(1-{[(4R,6S)-8-chloro-6-(2,3-dimethoxyphenyl)-4H,6H-pyrrolo[1,2-a][4,1]benzoxazepin-4-yl]acetyl}piperidin-4-yl)acetic 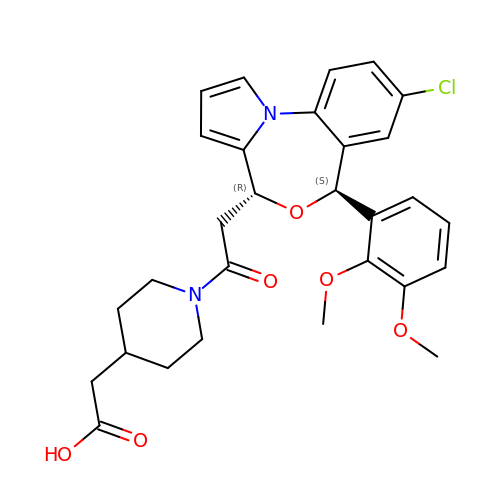acid | C29 H31 Cl N2 O6 | MSSQOQPKGAMUSY-LEAFIULHSA-N> GEDRRVPQNWFPIFNPERSDKPNASDPSVPLKIPLQRNVIPSVTRVLQQTMTKQQVFLLERWKQRMILELGEDGFKEYTSNVFLQGKRFHEALESILSPQETLKERDENLLKSGYIESVQHILKDVSGVRALESAVQHETLNYIGLLDCVAEYQGKLCVIDWKTSEKPKPFIQSTFDNPLQVVAYMGAMNHDTNYSFQVQCGLIVVAYKDGSPAHPHFMDAELCSQYWTKWLLRLEEYTEKKKNQNIQKPEYS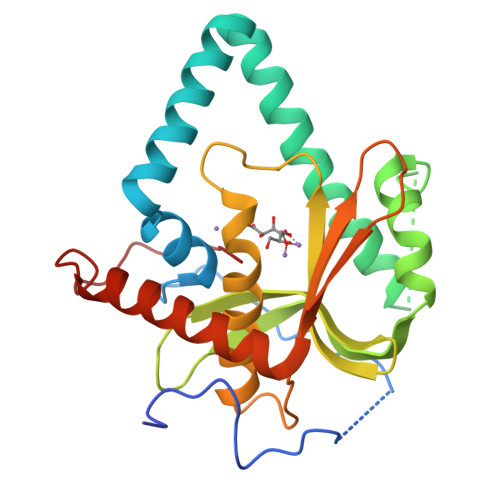E>MPLDPRIKELLESGFIVPIGKASVDEVRKIFRQLASAAPKVEVGKVEDIKIPGSEANINARVYLPKANGPYGVLIYLHGGGFVIGDVESYDPLCRAITNACNCVVVSVDYRLAPEYKFPSAVIDSFDATNWVYNNLDKFDGKMGVAIAGDSAGGNLAAVVALLSKGKLNLKYQILIYPAVGFDSVSRSMIEYSDGFFLTREHIEWFGSQYLRSPADLLDFRFSPILAQDLSGLPPALIITAEYDPLRDQGEAYANRLLQAGVPVTSVRFNNVIHGFLSFFPLIEQGRDAISLIGSVLRRTFYDKSAAAHH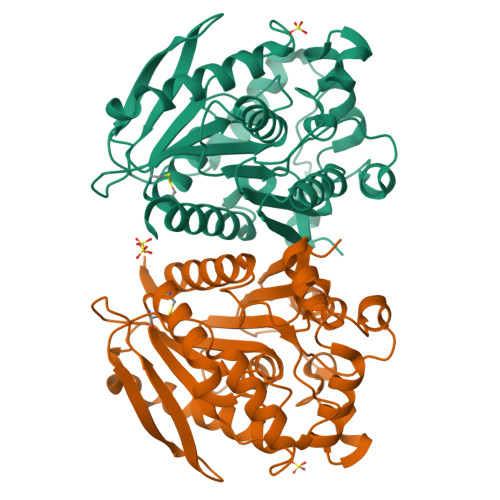HHHH[4x]3-azanyl-3-(hydroxymethyl)-1,5,7,11-tetraoxa-6$l^{4}-boraspiro[5.5]undecan-9-ol 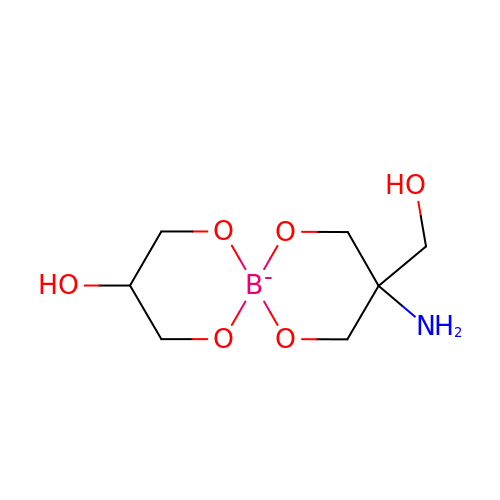| C7 H15 B N O6 | NORKYMYNBIQBFM-FXQIFTODSA-N7-BENZYL GUANINE 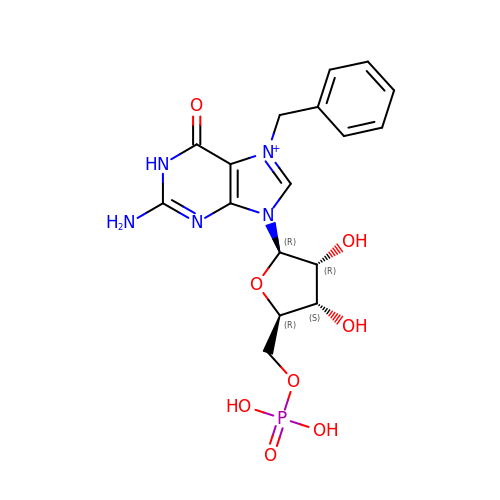MONOPHOSPHATE | C17 H21 N5 O8 P | WMKJRKYLDWLLPS-XNIJJKJLSA-O> MADLNWETVISSDSSPAVENEHPQETPESNNSVYTSFMKSHRCYDLIPTSSKLVVFDTSLQVKKAFFALVTNGVRAAPLWDSKKQSFVGMLTITDFINILHRYYKSALVQIYELEEHKIETWREVYLQDSFKPLVCISPNASLFDAVSSLIRNKIHRLPVIDPESGNTLYILTHKRILKFLKLFITEFPKPEFMSKSLEELQIGTYANIAMVRTTTPVYVALGIFVQHRVSALPVVDEKGRVVDIYSKFDVINLAAEKTY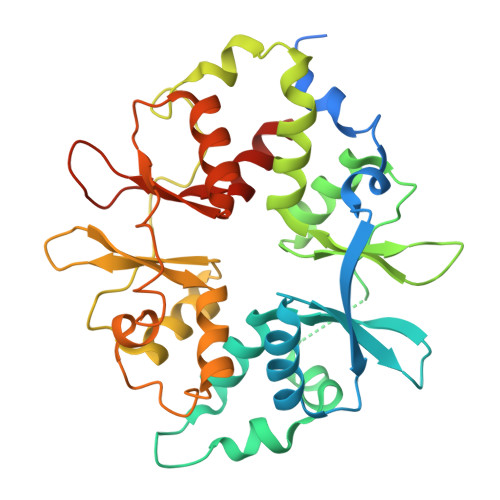NNLDVSVTKALQHRSHYFEGVLKCYLHETLETIINRLVEAEVHRLVVVDENDVVKGIVSLSDILQALVLTGGEKKP> SMTNVQILHGDLSPDLCDLAR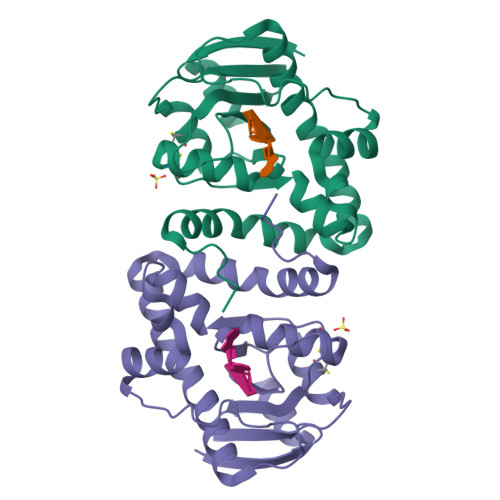ASELVGWDIETSGLDWRNGQIGTCQLAIGDSVAVVVLGDDDHPQGLCDLLADDGVRKIFHHAPFDIRFMAQQWDCKPRNLACTKIASKVLNPSAEHATHSLKPLLKATLGVDIDKGQQQSSWTTGVLTAEQMSYAVSDVVYLSELYSQLRAQCLDKGVLQAVENAYSFLPVWVELQRRGIEDVFAY>[7x]MSRVPSPPPPAEMSSGPVAESWCYTQIKVVKFSYMWTINNFSFCREKMGEVIKSSTFSSGANDKLKWCLRVNPKGL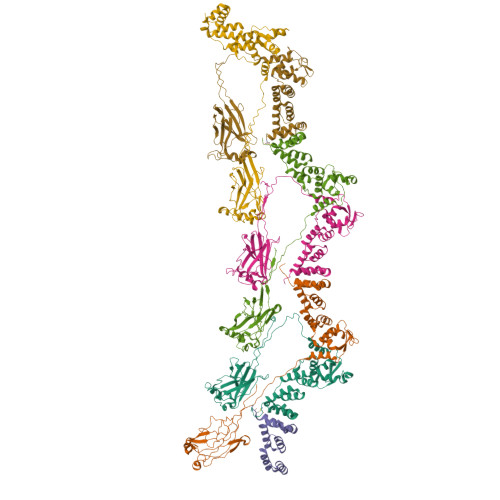DEESKDYLSLYLLLVSCPKSEVRAKFKFSILNAKGEETKAMESQRAYRFVQGKDWGFKKFIRRDFLLDEANGLLPDDKLTLFCEVSVVQDSVNISGQNTMNMVKVPECRLADELGGLWENSRFTDCCLCVAGQEFQAHKAILAARSPVFSAMFEHEMEESKKNRVEINDVEPEVFKEMMCFIYTGKAPNLDKMADDLLAAADKYALERLKVMCEDALCSNLSVENAAEILILADLHSADQLKTQAVDFINYHASDVLETSGWKSMVVSHPHLVAEAYRSLASAQCPFLGPPRKRLKQS Trx is a small cytoplasmic enzyme that can reduce di­sulfide bonds in various cellular proteins. Trx has a common CxxC motif (C: cysteine; x: small hydro­phobic residue) in the active site, and this motif is critical to its reductase activity. The most distinct difference between the two Trxs is Trx2’s possession of an additional 30–40 residues at the N-terminus, which forms a zinc-binding motif using four conserved cysteine residues. A. baumannii contains both Trx1 (hereafter abTrx1) and Trx2 (hereafter abTrx2).

Finally, the 1.20 Å high-resolution crystal structure of abTrx2 was solved with the MR phasing method. Interestingly, although abTrx2 was purified and crystallized in an oxidized state, the CxxC redox center of abTrx2 is in a reduced form, characterized by the absence of a di­sulfide-bond between the two cysteine residues at the CxxC motif. The structure of abTrx2 is most closely related to that of rcTrx2, which has a reduced form of the CxxC motif. Pairwise structural alignments of abTrx2 with the three structural homologues show that only abTrx2 has an α1 helix at the zinc-finger domain [Figs. 3(c)–3(e)]. Although the number of reported Trx2 structures is limited, this structural difference may indicate that the Trx2 zinc-finger domain may be rotatable. According to the DTNB reduction assay, abTrxR showed strong TrxR activity in the presence of purified abTrx1 or abTrx2. However, the abTrx2 C28V variant completely lost its TrxR activity, while TrxR in the R13E variant decreased by almost half [Fig. 4(e)].

> GSHMMIIVCASCDAKNRVPEEKLTAQPSCGQCHQPLLPLEPIELNEQNFSNYITNSDLPILIDLWAEWCGPCKMMAPHFAQVAKQNPRVIFAKINTEESPRLSQAFNVRSIPTLVLMNKTTEVARMSGALRAPELQQWLDQQLQTNFGS>[2x]AKHPDSVIYQTSLMSALLSGVYEGDTTIADLLAHGDFGLGTFNELDGEMIAFSSQVYQLRADGSARAAKPEQKTPFAVMTWFQPQYRKTFDAPVSRQQIHDVIDQQIP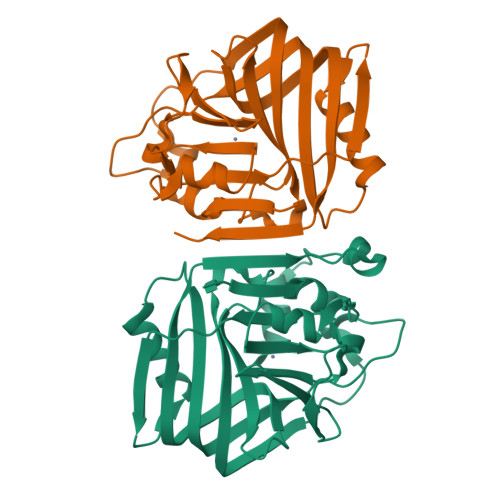SDNLFCALRIDGNFRHAHTRTVPRQTPPYRAMTDVLDDQPVFRFNQREGVLVGFRTPQHMQGINVAGYHEHFITDDRQGGGHLLDYQLESGVLTFGEIHKLMIDLPADSAFLQANLHPSNLDAAIRSVEN> MVNAEDLFINLAKSLLGDDVIDVLRILLDKGTEMTDEEIANQLNIKVNDVRKKLNLLEEQGFVSYRKTRDKDSGWFIY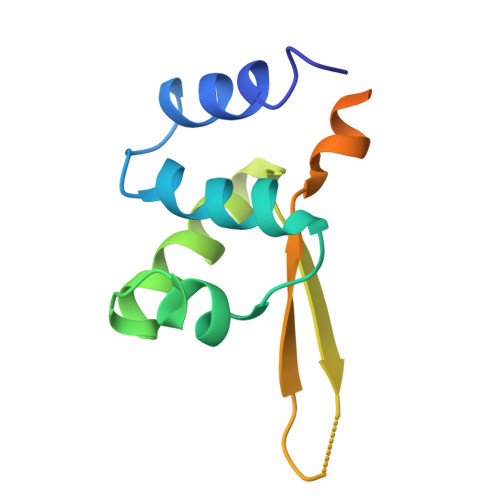YWKPNIDQINEILLNRKRLILDKLKTRLEYEK>MRGSHHHHHHIAASTLDEIMKRGTLRVGTDADYKPFSFKDKNGQYTGFDIDLAKALAKELGVKVEFVPTTWDGIIPALQTGKFDIVMSGMTITPERKKKVDFSDPYMTAGQTILVKKDNADKIKSFEDLNKPD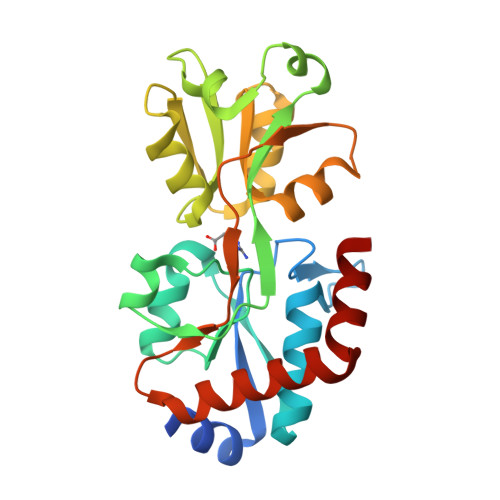VKVAVQLGTTSEQAAKEFLPKAKIRTFENNAEAFQEVVSGRADAMVTDSPVAAYYAKKNPGLAVVVVDEPFTHEPLGFAIRKGDPELLNWVNNWLKQMKKDGTYDKLYEKWFKL[4x]3-(2-chlorophenyl)-N-[(1R)-1-(3-methoxyphenyl)ethyl]propan-1-amine 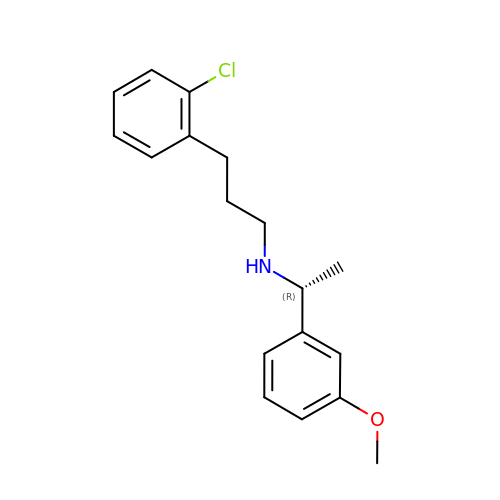| C18 H22 Cl N O | ZVQUCWXZCKWZBP-CQSZACIVSA-N>MQKETVIIIGGGPCGLAAAISLQKVGINPLVIEKGNIVNAIYNYPTHQTFFSSSEKLEIGDVAFITENRKPVRNQALAYYREVVRRKSVRVNAFERVEKVQKDGEAFQVETTKRDGSKEIYIAKYIVVATGYYDNPNYMNVPGEELKKVAHYFKEGHPYFDRDVVVIGGKNSSVDAALELVKSGARVTVLYRGIEYSPSIKPWILPEFEALVRNGTIQMHFGAHVKEITEHTLTFTVDGEALTIKNDFVFAMTGYHPDHSFLTKMGVQIDEETGRPFYTEDRMETNAENIFIAGVIAAGN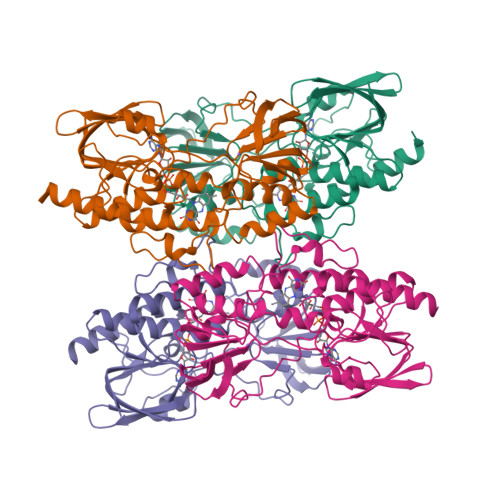NANEIFIENGRFHGDAIAQTIASREK[4x]> MADSNLNEPVIIQATRLD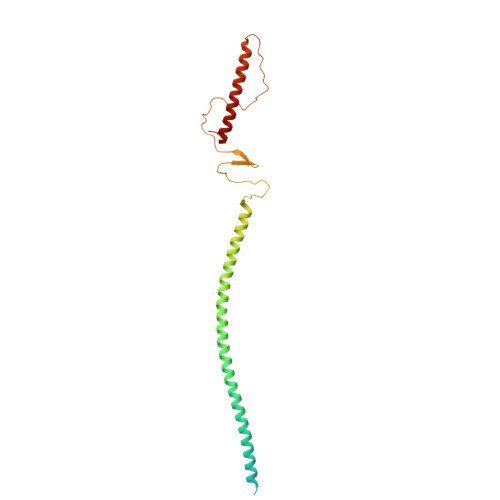TSILPRNIFSQSYLLYVIAQGTDVGNVANKANEAGQGAYDAQVKNDEQDVELADHDARIAANTKAINILEVRLTTAEGKIVVLRSDVDYLLDEVIDIQAHLVTVDQRLDGVESDVSDIKSDYVSKTVTESQSLASPLDVKTSYSVDGIQVVGARQTGWTAATGTPLLGSFNANQSYTVGTTYTQSEVAALATGLEQARQRILALETALRLHGLID4-azanyl-3-[(2~{S},3~{R},4~{S},5~{R})-3,4-bis(oxidanyl)-5-(phosphonooxymethyl)oxolan-2-yl]-1~{H}-pyrazole-5-carboxylic 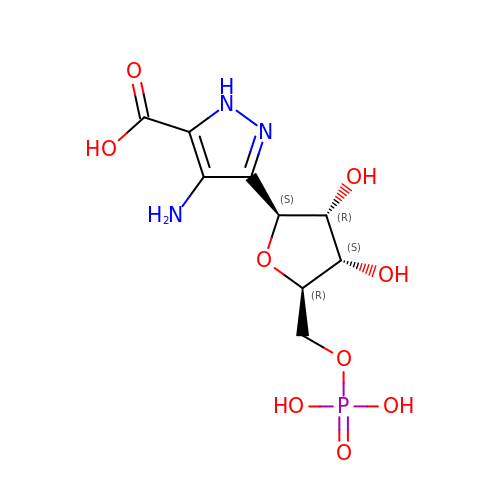acid | C9 H14 N3 O9 P | KFBPDQGSYVBBLS-UOQNBVRUSA-N>[2x]AGHMKQRFIRQFTNLMSTSRPKVVANKYFTSNTAKDVWSLTNEAAAKAANNSKNQGRELINLGQGFFSYSPPQFAIKEAQKALDIPMVNQYSPTRGRPSLINSLIKLYSPIYNTELKAENVTVTTGANEGILSCLMGLLNAGDEVIV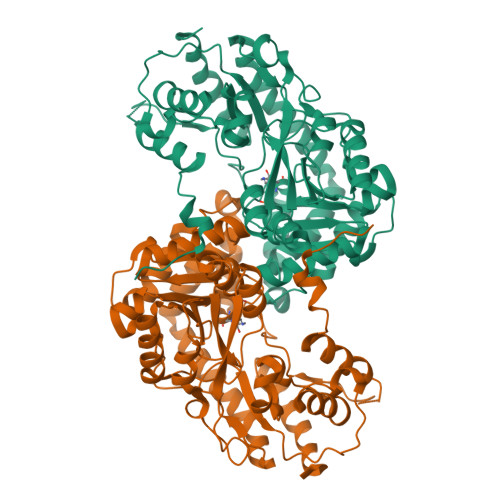FEPFFDQYIPNIELCGGKVVYVPINPPKELDQRNTRGEEWTIDFEQFEKAITSKTKAVIINTPHNPIGKVFTREELTTLGNICVKHNVVIISDEVYEHLYFTDSFTRIATLSPEIGQLTLTVGSAGKSFAATGWRIGWVLSLNAELLSYAAKAHTRICFASPSPLQEACANSINDALKIGYFEKMRQEYINKFKIFTSIFDELGLPYTAPEGTYFVLVDFSKVKIPEDYPYPEEILNKGKDFRISHWLINELGVVAIPPTEFYIKEHEKAAENLLRFAVCKDDAYLENAVERLKLLKDYL>PLREAKDLHTALHIGPRALSKACNISMQQAREVVQTCPHCNSAPALEAGVNPRGLGPLQIWQTDFTLEPRMAPRSWLAVTVDTASSAIVVTQHGRVTSVAVQHHWATAIAVLGRPKAIKTDNGSCFTSKSTREWLARWGIAHTTGIPGNSQGQAMVERANRLLKDKIRVLAEGDGFMKR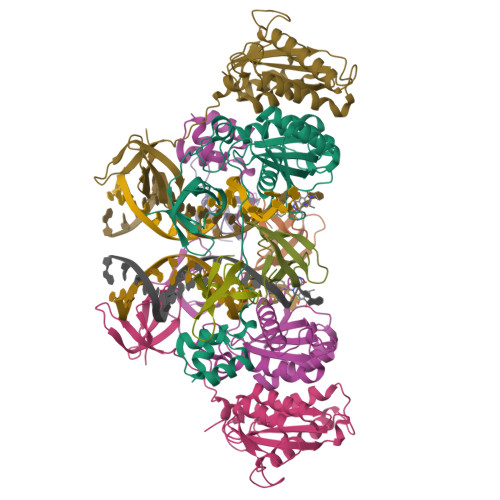IPTSKQGELLAKAMYALNHFERGENTKTPIQKHWRPTVLTEGPPVKIRIETGEWEKGWNVLVWGRGYAAVKNRDTDKVIWVPSRKVKPDITQKDEVTKK[8x]>GSPCELLPVGVGHPVQAMLKSFTALSGCASRGT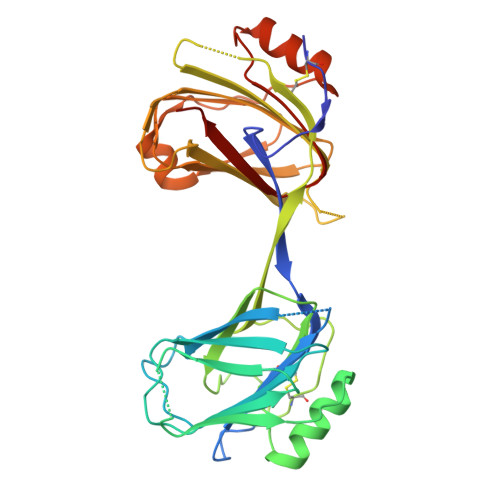TSHPQEVHIINLRKGSAQGAREKTAEVALHLRPIQSLHVHQKPLVFILNSPQPILWKVRTEKLAPGVKRIFHVVEGSEVHFEVGNFSKSCEVKVETLPHGNEHLLNWAHHRYTAVTSFSELRMAHDIYIKVGEDPVFSETCKIDNKFLSLNYLASYIEPQPSTGCVLSGPDHEQEVHIIELQAPNSSSAFQVDVIVDLRPLDGDIPLHRDVVLLLKCEKSVNWVIKAHKVMGKLEIMTSDTVSLSEDTERLMQVSKTVKQKLPAGSQALIQWAEENGFNPVTSYTNTPVANHFNLRLREHHHHHH[2x]> SNQYQLPLNVRPYTTTWCSQSPSCSNLLAIGHDTGITIYCASEEQTPGSTGLTLQELFTIQTGLPTLHLSFSSSCSYSENLHDGDGNVNSSPVYSLF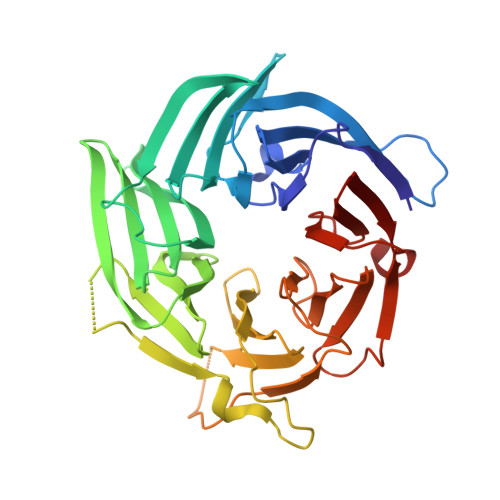LACVCQDNTVRLIITKNETIITQHVLGGKSGHHNFVNDIDIADVYSADNRLAEQVIASVGDDCTLIIWRLTDEGPILAGYPLSSPGISVQFRPSNPNQLIVGERNGNIRIFDWTLNLSAEENSQTELVKNPWLLTLNTLPLVNTCHSSGIASSLANVRWIGSDGSGILAMCKSGAWLRWNLFANNDYNEISDSTMKLGPKNLLPNVQGISLFPSLLGACPHPRYMDYFATAHSQHGLIQLINTYEKDSNSIPIQLGMPIVDFCWHQDGSHLAIATEGSVLLTRLMGFT> MIKKAVLPVAGLGTRFLPASKSIPKEMVTVVDRPAIEYVVREAVEAGIEQIILVTHSSKASIENYFDRNFELETTLEQKKKFDLLAEITQIVE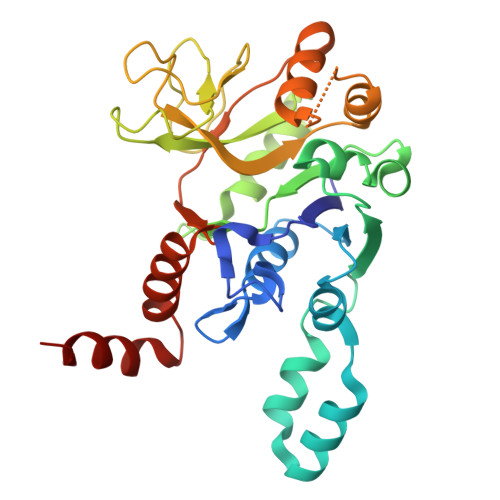EHVSVISVRQPQPLGLGHAVLCAKSVVGEDDFAVLLPDVLVKDGSGQNDLSRMISRYNSSQAAQIMVEAVPDHLVDQYGIVDVAQSPNEGESIAMQGIVEKPPVGAAPSNLSVVGRYVLPAKIMQLLENTPKGAGNEIQLTDAIAMLQDTDTVEAYRMQGQTFDCGSKLGYLKAVLHYGLEHPKLGMEFKQLILELK1-(5'-PHOSPHO-BETA-D-RIBOFURANOSYL)BARBITURIC ACID | C9 H13 N2 O10 P | 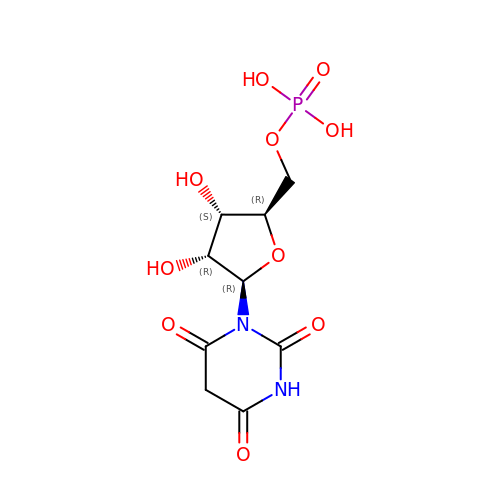AODYJUNLDJOADV-YXZULKJRSA-N>AECSVDIQGNDQMQFNTNAITVDKSCKQFTVNLSHPGNLPKNVMGHNFVLSTAADMQGVVTDGMASGLDKDFLK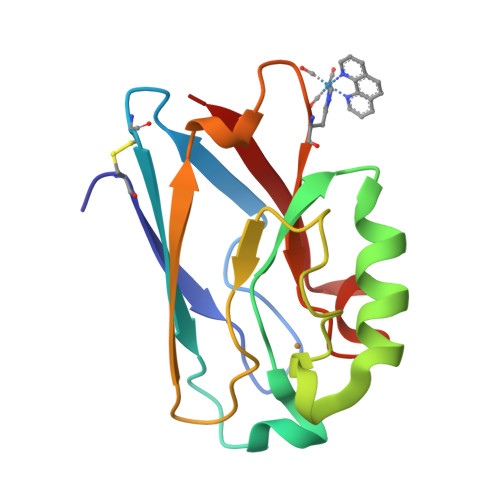PDDSRVIAQTKLIGSGEKDSVTFDVSKLKEGEHWMFFCTFPGHSALMKGTLTLK[4x]> ASCPGACVCYNEPKVTTSCPQQGLQAVPTGIPASSQRIFLHGNRISHVPAASFQSCRNLTILWLHSNALARIDAAAFTGLTLLEQLDLSDNAQLHVVDPTTFHGLGHLHTLHLDRCGLRELGPGLFRGLAALQYLYLQDNNLQALPDNTFRDLGNLTHLFLHGNRIPSVPEHAFRGLHSLDRLLLHQNHVARVHPHAFRDLGRLMTLYLFANNLSMLPAEVLMPLRSLQYLRLNDNPWVCDCRARPLWAWLQKFRGSSSE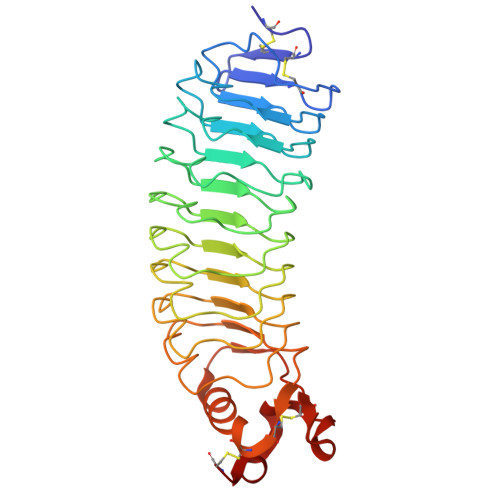VPCNLPQRLADRDLKRLAASDLEGC> MPSFDIVSEVDLQEARNGVDNAVREVESRFDFRGVEATIELNDANKTIKVLSESDFQVNQLLDILRAKLLKRGIEGASLDVPDEFVHSGKTWYVEAKLKQGIESAVQKKIVKLIKDSKLKVQAQIQGEEIR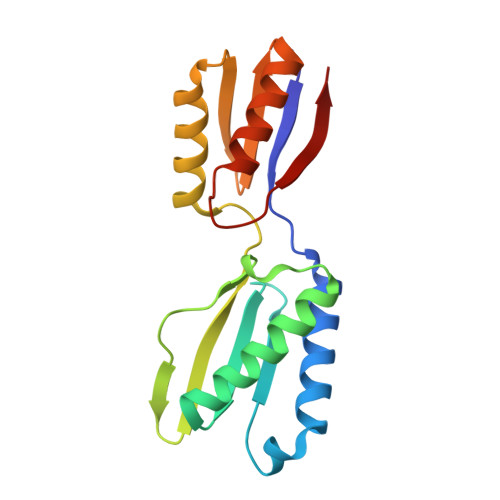VTGKSRDDLQSVMALVRGGDLGQPFQFKNFRD>[6x]GPMFEARLVQGSILKKVLEALKDLINE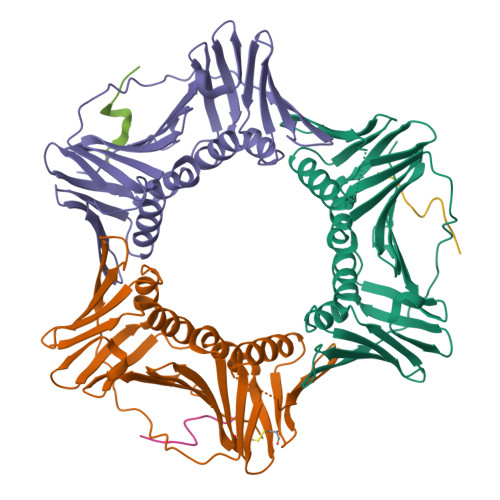ACWDISSSGVNLQSMDSSHVSLVQLTLRSEGFDTYRCDRNLAMGVNLTSMSKILKCAGNEDIITLRAEDNADTLALVFEAPNQEKVSDYEMKLMDLDVEQLGIPEQEYSCVVKMPSGEFARICRDLSHIGDAVVISCAKDGVKFSASGELGNGNIKLSQTSNVDKEEEAVTIEMNEPVQLTFALRYLNFFTKATPLSSTVTLSMSADVPLVVEYKIADMGHLKYYLAPKIEDEEGS;>MEQRRVTDFFARRR[6x]>[6x]MLEAQVQFASLWKRLVECINGLVNEANFDCNPGGLSVQAMDSSHVALVHMLLRDDCFVKYQCGRNSILGLNLASLSKVLKIVDSND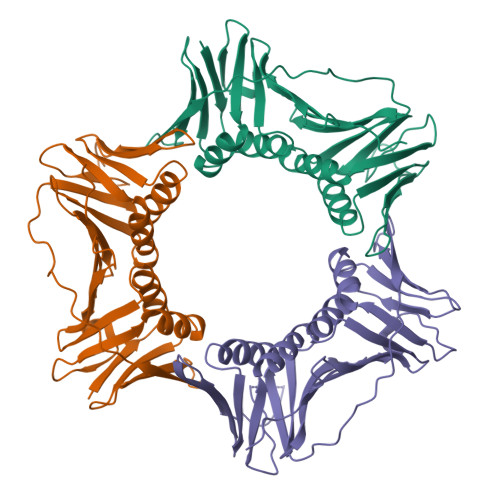SLSLRHDDDSDVVTLTSENPEKTRKCEYQLKLLEIEAESMGIPEMDYRSTVTLNSAEFAKIVRDMQVFGDTVTIAISKEGVKFSSSGDVGQGYTFLQAAGVSDRSTKGVEVTMEEPITLSFALRFMGIFAKGSTLSERVTLKFAKDSPCMVEYGIDNVGYLRYYLAPKVDDAE> SPSAEECGYSDRVRSITLGNSTITTQECANVVVGYGVWPTYLNDDEATAEDQPTQPDVATCRFYTLESVMWQQSSPGWWWKFPDALSNMGLFGQNMQYH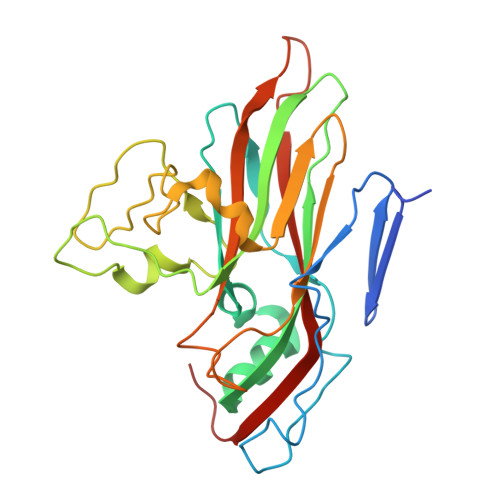YLGRAGYTVHVQCNASKFHQGCLLVVCVPEAEMGCATLANKPDQKSLSNGETANMFESQNSTGQTAVQANVINAGMGVGVGNLTIFPHQWINLRTNNSATIVMPYINSVPMDNMFRHNNFTLMIIPFAPLSYSTGATTYVPITVTVAPMCAEYNGLRLAGKQ> IPTSIDWRQKGAVTPVRNQGGCGSCWTFSSVAAVEGINKIVTGQLLSLSEQELLDCERRSYGCRGGFPLYALQYVANSGIHLRQYYPYEGVQRQCRASQAKGPKVKTDGVGRVPRNNEQALIQRIAIQPVSIVVEAKGRAFQNYRGGIFAGPCGTSIDHAVAAVGYGNDYILIKNSWGTGWGEGGYIRIKRGSGNPQGACGVLSDSVF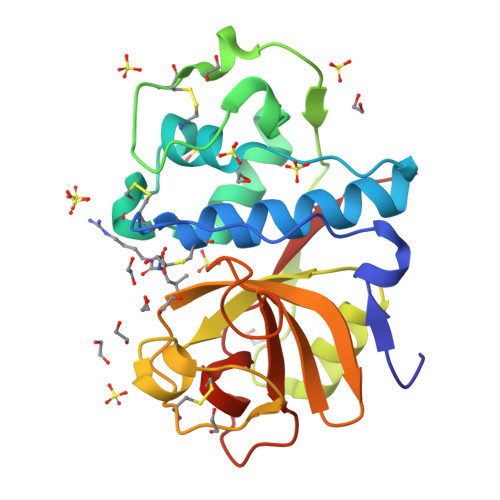PTKNR> SPSAEACGYSDRVAQLTIGNSTITTQEAANIIVGYGEWPSYCSDDDATAVDKPTRPDVSVNRFYTLDTKLWEKSSKGWYWKFPDVLTETGVFGQNAQFHYLYRSGFCIHVQCNASKFHQGALLVAILPEYVIGTVAGGTGTEDSHPPYKQTQPGADGFELQHPYVLD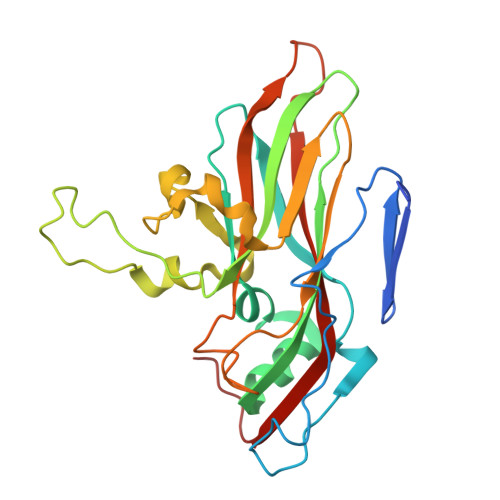AGIPISQLTVCPHQWINLRTNNCATIIVPYMNTLPFDSALNHCNFGLLVVPISPLDFDQGATPVIPITITLAPMCSEFAGLRQAVTQ> MAEANLDKKPEVKPPPGLKAIIDHLGQVYPNQPNPLQVTTLLKYWLGGQDPLDYISMYNYPGDVDRNVPPHWHYISFGLSDLHGDERVH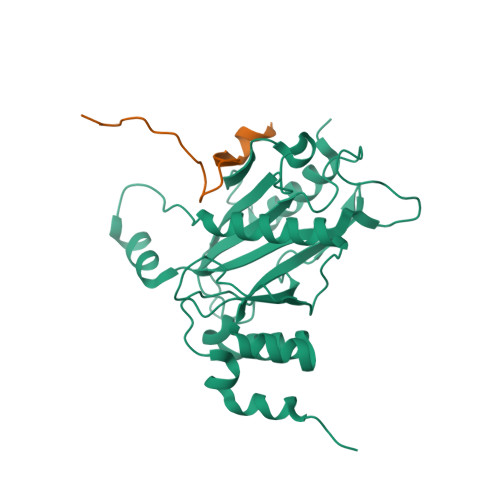LREEGVTRSGMGFELTFRLAKTEIELKQQIENPEKPQRPPTWPANLLQAIGRYCFQTGNGLCFGDNIPWRKSLDGSTTSKLQNLLVAQDPQLGCIDTPTGTVDFCQIVGVFDDELEQASRWNGRGVLNFLRQDMQTGGDWLVTNMDRQMSVFELFPETLLNLQDDLEKQ;> AAPVINSHTCFVSGNSNMILNHMNDNFA In this paper we describe the first crystal structure of CNMT, an essential enzyme in the core pathway to BIAs, which introduces the amino methyl functionality that is often essential for the bioactivity of most of the medically important BIAs. Previous studies with CNMT from Coptis japonica showed that this S‐adenosyl‐l‐methionine (AdoMet) dependent enzyme can N‐methylate a number of natural THIQ, exhibiting highest activity with coclaurine 4 and heliamine 8.8 To further characterize this enzyme, the C. japonica CNMT was overproduced in E. coli. The CNMT structure reveals a typical class I methyltransferase α/β Rossmann fold forming the AdoMet‐binding domain, which is capped by a predominantly alpha helical BIA substrate recognition domain. CNMT forms a dimeric interface made up of 13 hydrogen bonds and 3 salt bridges, similar to that seen in the PavNMT structure.

The structure of CNMT with 9 is very similar to the N‐methylheliamine 8 a structure except the two ligands are flipped relative to one another in the active site, with the carbonyl group of 9 in the same position as the amino group of 8 a.

>QTKKAAIVELLKQLELGLVPYDDIKQLIRRELARRLQWGYKPTYEEQIAEIQNLTHSLRQMKIATEVETLDSQLYEIPIEFLKIMNGSNLKGSCCYFKEDSTTLDEAEIAMLDLYCERAQIQDGQSVLDLGCGQGALTLHVAQKYKNCRVTAVTNSVSQKEYIEEESRRRNLLNVEVKLADITTHEMAETYDRILVIELFEHMKNYELLLRKISEWISKDGLLFLEHICHKTFAYHYEPLDDDDWFTEYVFPAGTMIIPSASFFLYFQDDVSVVNHWTLSGKHFSRTNEEWLKRLDANLDVIKPMFETLMGNEEEAVKLINYWRGFCLSGMEMFGYNNGEEWMASHVLFKK[2x]>TTNDTYEATYAIPMHCENCVNDIKACLKNVPGINSLNFDIEQQIMSVESSVAPSTIINTLRNCGKDAIIRGAGKPNSSAVAILETFQKYTIDQKKDTAVRGLARIVQVGENKTLFDITVNGVPEAGNYHASIHEKGDVSKGVESTGKVWHKFDEPIECFNESDLGKNLYSGKTFLSAPL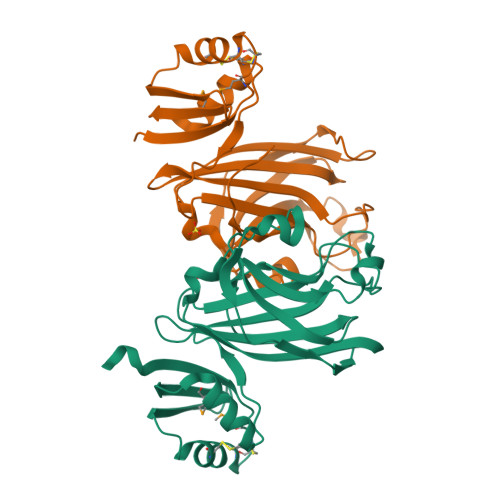PTWQLIGRSFVISKSLNHPENEPSSVKDYSFLGVIARSAGVWE[2x]>MGSHHHHHHSSGLEVLFQGPAEAKKEIPLKYGATNEGKRQDPAMQKFRDNRLGAFIHWGLYAIPGGEWNGKVYGGAAEWLKSWAKVPADEWLKLMDQWNPTKFDAKKWAKMAKEMGTKYVKITTKHHEGFCLWPSKYTKYTVANTPYKRDILGELVKAYNDEGIDVHFYFSVMDWSNPDYRYDIKSKEDSIAFSRFLEFTDNQLKELATRYPTVKDFWFDGTWDASVKKNGWWTAHAEQMLKELVPGVAINSRLRADDKGKRHFDSNGRLMGDYESGYERRLPDPVKDLKVTQWDWEACMTIPENQ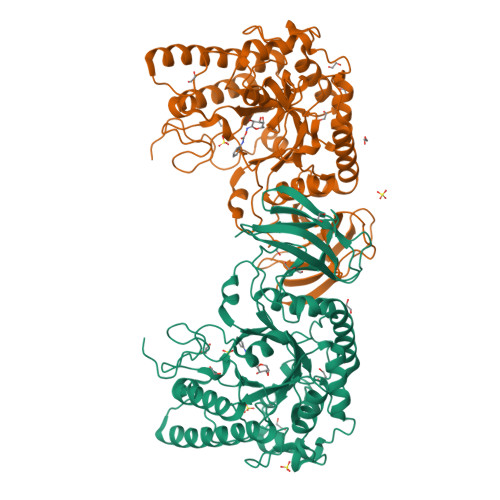WGYHKDWSLSYVKTPIEVIDRIVHAVSMGGNMVVNFGPQADGDFRPEEKAMATAIGKWMNRYGKAVYACDYAGFEKQDWGYYTRGKNDEVYMVVFNQPYSERLIVKTPKGITVEKATLLTTGEDITVVETTRNEYNVSVPKKNPGEPYVIQLKVRAAKGTKSIYRDALT[2x]>[2x]MNHKVHHHHHHLQENLYFQG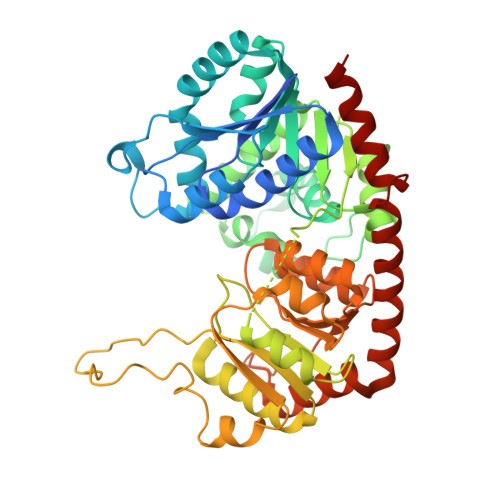MEMEAPLIVIVPSPGMGHLIPLVEFAKVLVSRFHFSVSLLLPTTAQPTKAQTTLLNSLPSSVSHNFLPTVDPAHLPDGVAHEVTISLTHAHSLSSIRAALGSLAQQAQVVALITDLFGTGLYTVARDLGIPPYLYFTSTAMCLLFLFHLPKLDETVSCEYRDMPEPLVLPGCVPLHGKDFVDPAQDRQDQAYHVLLDHVKRYVLAEGIFVNTFVDLEPGAIKTLQTEDPNVPPVYPVGPIIQSGLDDDSHGSDCLKWLDRQPSGSVLFVSFGSGGTLSNEQLNELAIGLEISGHRFLWVVRSPNDHSSFGSFFSTQSQDDPFGFLPTGFVDRIKDRGLLVPSWAPQIKVLSHGSTGGFLTHCGWNSTLESIVNGVPLIVWPLYAEQRMNAVMLNQGLKVALRPNASQRGLVEADEIARVVKELMDGDEGKKARYKMRELSDSAKRVTSENGESTKLLSEVASKWSQCKS N-valyl-histidine derived from proteolytic digestion of the N-terminus of the HbA1c β-chain. This study reports the X-ray structures of the wild-type and Asn56Ala (N56A) mutant of Phaeosphaeria nodorum fructosyl peptide oxidase (PnFPOX) to elucidate the residues responsible for the oxidative half-reaction. Fructosyl amine oxidases (FAOXs) are FAD-containing enzymes that catalyze the oxidative deglycosylation of fructosyl amino acids such as fructosyl valine and/or ε-fructosyl lysine, which are the degradation products of HbA1c and GA, respectively. As members of the FAOX family, fructosyl peptide oxidases (FPOXs) are also known as candidates for diagnostic enzymes. A covalent bond is formed between FAD and Cys343 of PnFPOX as observed in amadoriase I (Cys342), amadoriase II (Cys335), and EtFPOX (Cys347).

To investigate the oxygen binding site of PnFPOX, we attempted to soak NaCl into the crystals of wild-type and N56A PnFPOX, since the bound chloride side is considered an oxygen binding site in MSOX. The crystal of PnFPOX N56A with NaCl diffracted well and the structure was determined at 1.8 Å. Although bound chloride ions were found in the structure of PnFPOX N56A with NaCl, no chloride was bound at the W2 position. Oxygen was almost unable to bind at the position of W2. Therefore, we concluded that W2 could not be a putative oxygen binding site, but that the W2 position is in the plausible main oxygen accessible channel. N56A showed decreased oxidase activity compared to the wild -type, while its dye-mediated dehydrogenase activity was higher than that of wild type. Interestingly, in PnFPOX N56A, Lys274 cannot form a hydrogen bond with Ala56 but instead moves toward Asp54, forming salt bridges 2.92–3.35 Å in length. This movement results in the elimination of the water molecule from position W2, although Lys274 can interact with N5 of the isoalloxazine ring via a water molecule (W1, 2.81 Å from Lys274 and 3.11 Å from N5 of the isoalloxazine ring). The analysis of the protein channels of the structures showed that the W1, W2, and W4 positions in wild-type PnFPOX (W1′ and W4′ in PnFPOX N56A) are in the main oxygen-accessible channel. In PnFPOX N56A, the movement of Asp54 and Lys274 blocks a short and plausible main channel observed in wild-type PnFPOX (blue dotted path with arrow in Supplementary Figure S6). Although the oxygen could be accessible through another alternative long path instead of the closed path in PnFPOX N56A, the elimination of the accessibility toward the short pathway might result the drastic decrease in oxidase activity compared with dye-mediated dehydrogenase activity.

>[2x]MAPSRANTSVIVVGGGGTIGSSTALHLVRSGYTPSNVTVLDAYPIPSSQSAGNDLAKIMGVSLRNPVDLQLALEARQMWNEDELFKKFFHNTGRLDCAHGEKDIADLKSGYQALVDAGLDATNEWLDSEDEILKRMPLLSRDQIKGWKAIFSKDGGWLAAAKAINAVGEYLRDQGVRFGFYGAGSFKAPLLAEGVCIGVETVDGTRYYADKVVLAAGAWSPTLVELHEQCVSKAWVYGHIQLTPEEAARYKNSPVVYNGDVGFFFEPNEHGVIKVCDEFPGFTRFKMHQPFGAKAPKRISVPRSHAKHPTDTIPDASDVSIRRAIATFMPQFKNKKMFNQAMCWCTDTADAALLICEHPEWKNFVLATGDSGHSFKLLPNIGKHVVELLEGTLADDLAHAWRWRPGSGDALKSRRSAPAKDLADMPGWNHDKPRANLLEHHHHHH> SLTSKNQFYKPGMLVPVFSAAGLLKNGRYQFLLQQIETLSLLPTEQYAQLYEALVYRFVEFVQVLPIRLDEPLCSLMNEGLLRGVNS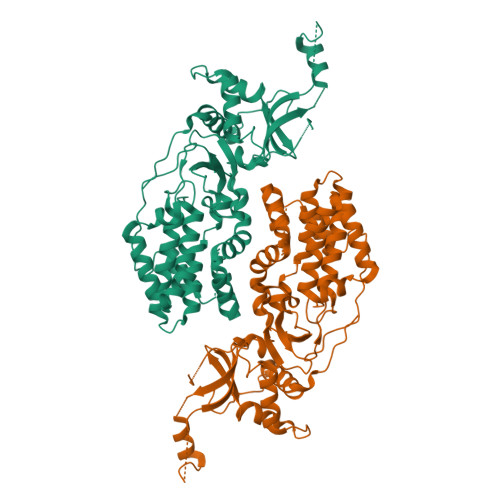LNHYIQNHPEATPLERYALFSAGLLLEVAHAVVNQKIFITDEEGNFIKQWNPFSGPLIDDVETKHYKIMPLSSYYQRNIPSITPILVRQLLPDEGFLWLTSDMRVFSDWMQALRDDEGEGGGRFEHVLQLFKHKNIDGLFNTLPALPVNLQDSPATAHADAFLNWLKEALATNQIKVNTSDAGVHVIPEGVFLEKTGIFKQYIDLHVNVPVNLFTVYQQFGNLFGLTKLSGIDYRFEQLFSEYPDALKRKSKMGFAGLIGIRRASPTREGVLIADPNLIFTRGEIPSATSYLKLSSAQKSQNIPMT N~2~-(6-aminohexyl)-N~2~-[(4-fluoro-3-methylphenyl)sulfonyl]-N-hydroxy-D-alaninamide | C16 H26 F N3 O4 S | 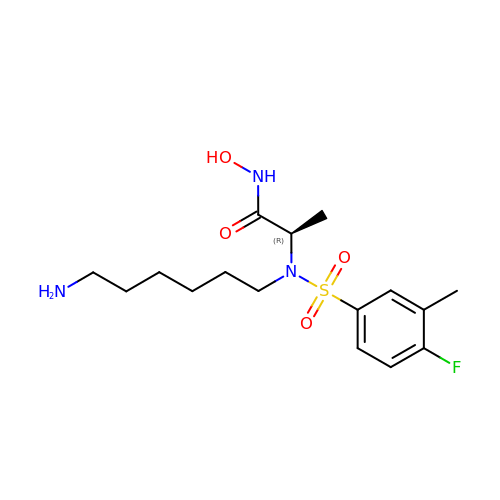GEZZNJHDANMDNY-CYBMUJFWSA-N>MDLGIQGKLAVVTAGSSGLGFASALELARNGARLLLFSRNREKLEAAASRIASLVSGAQVDIVAGDIREPGDIDRLFEKARDLGGADILVYSTGGP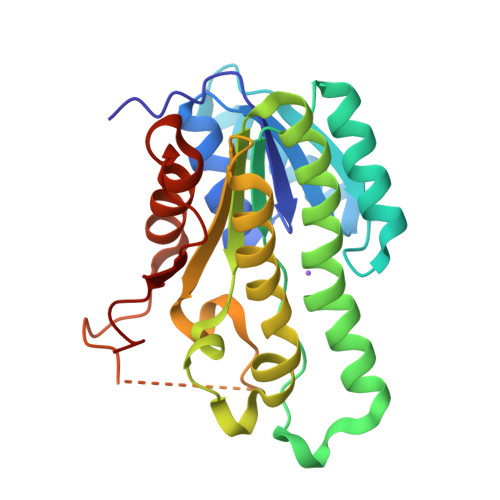RPGRFMELGVEDWDESYRLLARSAVWVGRRAAEQMVEKGWGRMVYIGSVTLLRPWQDLALSNIMRLPVIGVVRTLALELAPHGVTVNAVLPSLILTDRVRSLAEERARRSGITVEEALKSMASRIPMGRVGKPEELASVVAFLASEKASFITGAVIPVDGGAHI[2x]> MNITKPFPLPTGYFDIPLGLAALSLAWFHLENLFPAARMVSDVLGIVASAVWILFILMYAYKLRYYFEEVRAEYHSPVRFSFIALIPITTMLVGDILYRWNPLIAEVLIWIGTIGQLLFSTLRVSELW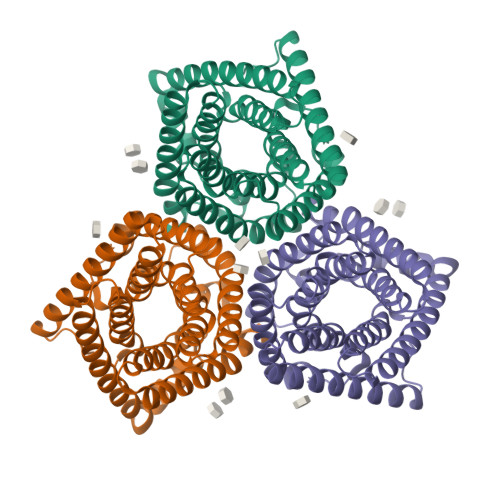QGGVFEQKSTHPSFYLPAVAANFTSASSLALLGYHDLGYLFFGAGMIAWIIFEPVLLQHLRISSLEPQFRATMGIVLAPAFVCVSAYLSINHGEVDTLAKILWGYGFLQLFFLLRLFPWIVEKGLNIGLWAFSFGLASMANSATAFYHGNVLQGVSIFAFVFSNVMIGLLVLMTIYKLTKGQFFLK> GSHMAKTVILDHDGNKDDFVAMILLLSNPKKVNLIGCICTDADCFVENGFDVTGKIMCAMHRLIKTPLFPIGKSTATAVNAFPTEWRFSAKNLDDMPFLNIVEDVALWEKLKPENEAHNGQQLLADLVMKSKEKVTVCVTGPLSNMAWCIEKYGEAFTSKVEECVIMGGAVDV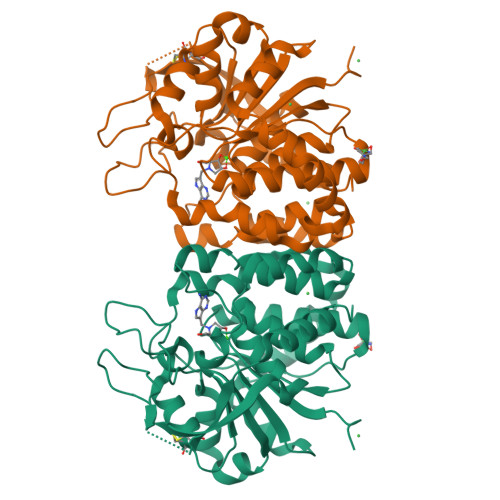GGNVFLPTTDGSAEWNIYWDPPAAKKVLCCPNIRCVLFSLDATNTVPVRSVDVKGFGAQNQYLLSQMVGTMWAMSTHEEILRDGDAYYAWDALTAAYILEPTIATLEPVALDVDVSKGKSEGRTPRASGEGKPCVHVARNPSKQMFHDLVFASTRVC> MRFRIRKCPKCGRYTLKETCPVCGEKTKVAHPPRFSPEDPYGEYRRRLKRELLGI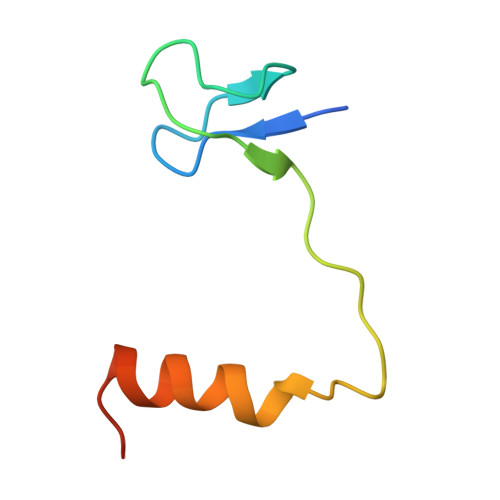GRKEK> TRMKNIECIELGRHRLKPWYFSPYPQELTTLPVLYLCEFCLKYGRSLKCLQRHLTKCDLRHPPGNEIYRKGTISFFEIDGRKNKSYSQNLCLLAKCFLDHKTLYYDTDPFLFYVMTEYDCKGFHIVGYFSKEKESTEDYNVACILTLPPYQRRGYGKLLIEFSYELSKVEGKTGTPEKPLSDLGLLSYRSYWSQTILEILMGLK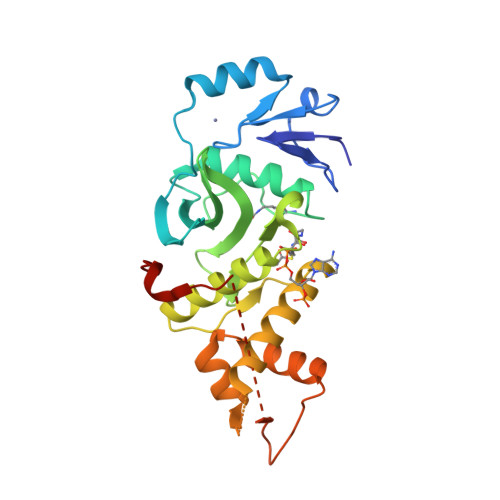SESGERPQITINEISEITSIKKEDVISTLQYLNLINYYKGQYILTLSEDIVDGHERAMLKRLLRIDSKCLHFTPKD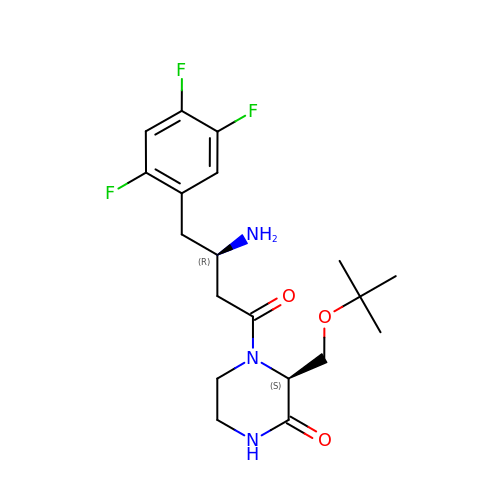(S)-4-((R)-3-amino-4-(2,4,5-trifluorophenyl)butanoyl)-3-(tert-butoxymethyl)piperazin-2-one | C19 H26 F3 N3 O3 | LCDDAGSJHKEABN-WBMJQRKESA-N> MVLIDYSKLSKEVAYALRHAPWEYGLELDAEGWVDINQLLSSLHECEKWKKVSEHDLHVMIEKSDKKRYEISNGKIRALYGHSIPQRIIKEQKCPPEVLYHGTARRFVKSIKEKGLQPQGRQYVHL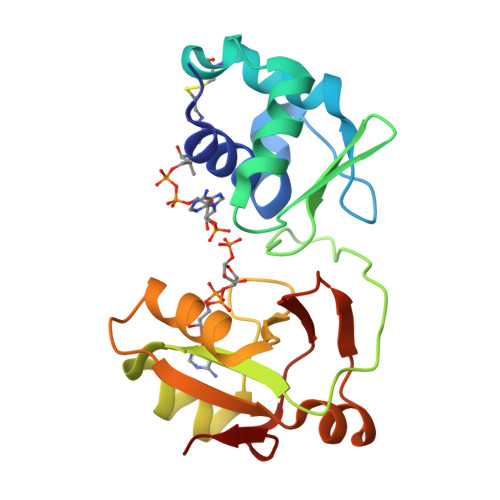SADVETALQVGKRRDIKPVLLIVNALEAWSEGIKFYLGNDKVWLADAIPSKYIRFE> MVSSKKFNQVDKGRGMISENYIEPAFLLPDLIEIQRSSFRWFLEEGLIEELNSFSPITDYTGKLELHFLGHNYKLKEPKYSVEEAKRRDSTYAVQMYVPTRLLNKETGDIKEQEVFIGDLPLMTDRGTFIINGAERVIVNQIVRSPGVYYKSEIDKNGRRTYSASLIPNRGAWLKFETDRNDLVWVRIDKTRKLSAQVLLKALGLSDNEIFDALRHPEYFQKTIEKEGQFSEEEALMELYRKLRPGEPPTVLGGQQLLDSRFFDPKRYDLGRVGRYKLNKKLRLSVPDTVRVLTSGDILAAVDYLINLEYDIGSIDDIDHLGNRRVRSVGELLQNQVRVGLNRLERIIRERMTVSDAEVLTPASLVNPKPLVAAIKEFFGSSQLSQFMDQTNPLAELTHKRRLSALGPGGLTRERAGFAVRDIHPSHYGRICPIETPEGPNAGLIGSLATHARVNQYGFLETPFRPVENGRVRFDQPAAYMTADEEDDLRVAPGDIPVDENGYIIGPQVPVRYRQEFSTTTPEQVDYVA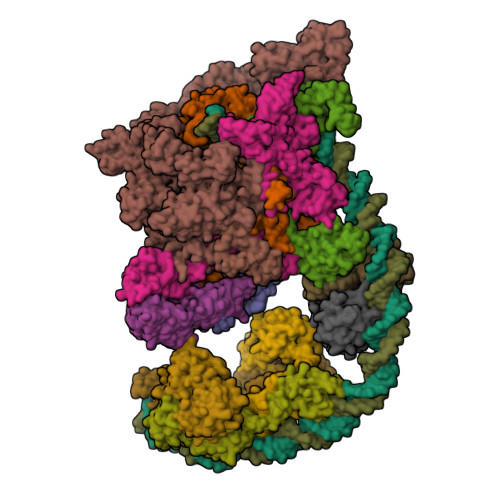VSPVQIVSVATSMIPFLEHDDANRALMGSNMQRQAVPLLKPERPLVGTGLEAQGARDSGMVIVSRTDGDVVYVDATEIRVRVSGQLPTASGKSTDNGQLTSQKGQEIRYTVSKYQRSNQDTCLNQKPLVRIGERVVAGQVLADGSSTEGGELALGQNIVVAYMPWEGYNYEDAILISERLVQDDIYTSIHIEKYEIEARQTKLGPEEITREIPNVGEDALRQLDEQGIIRIGAWVEAGDILVGKVTPKGESDQPPEEKLLRAIFGEKARDVRDNSLRVPNGEKGRVVDVRLFTREQGDELPPGANMVVRVYVAQKRKIQVGDKMAGRHGNKGIISRILPIEDMPYLPDGSPVDIVLNPLGVPSRMNVGQVFECLLGWAGHTLGVRFKITPFDEMYGEESSRRIVHGKLQEARDETGKDWVYNPDDPGKIMVYDGRTGEAFDRPVTIGVAYMLKLVHLVDDKIHARSTGPYSLVTQQPLGGKAQQGGQRFGEMEVWALEAFGAAYTLQELLTVKSDDMQGRNEALNAIVKGKAIPRPGTPESFKVLMRELQSLGLDIAVHKVETQADGSSLDVEVDLMADQLARRTPPRPTYESLSRESLDDDE;> MIFRNRVVDKGQLRNLISWAFTHYGTARTAVMADKLKDLGFRYATRAGVSISVDDLMVPPSKRSLLEAAEEEIRATEVRYQRGEITEVERFQKVIDTWNGTSEALKDEVVTHFKQTNPLNSVYMMAFSGARGNISQVRQLVGMRGLMADPQGEIIDLPIKTNFREGLTVTEYIISSYGARKGLVDTALRTADSGYLTRRLVDVSQDVIIREIDCGTTRGIPVRPMTEGSKTLIKLSTRLLGRVVGEDVIHPKTKEVIAPRNTPISDDLAKEIEKAGVAEVVVRSPLTCEAARSVCQHCYGWSLAHAKMVDLGEAVGIIAAQSIGEPGTQLTMRTFHTGGVFTGEVAQQVRSKMDGTIKLPRKLRTRTHRTRHGEDALFVESNGIMILEPRKEGSETPAPQEIHVTQGSTIYIVDGQQVKKGQLLAEVALGGRTTRTNTEKAVKDVASDLAGEVKFAEVVPEQKTDRQGNTTTTAARGGLIWILSGEVYNLPPGAELVVKNGDRVETNGVLAETKLTTIHGGVVRLPEATPGKSTREIEIITASVVLDQATVTVQSSQGRNNYLITTGNNQVFNLRATPGTKVQNGQVVAELIDDRYRTTTGGFLKFAGVEVQKKGKAKLGYEVVQGGTLLWIPEETHEVNKDISLLLVEDGQYVEAGTEVVKDIFCQNSGVVEVTQKNDILREVVVKPGELLMVDDPEAVIGRDNTLLQPGEELLGQVATELRYIQYVESPEGPALLSRPVVEFAVPSNPDVPSTTSVSQQTGRSIQMRAVQRLPYKDSERVKSVEGVELLRTQLVLEIEQEGEQEHNASPLAADIELIPDLEDADVQRLQLVILESLVLRRDIAADATQGSTQTSLEVKDGDTIVPGSVVARTQILSKEGGIVRGVQKGSEAVRRCLVLRHSDMATLNISAKPKVKAGDLIVAGTELAPGIFAEESGQIVGVKNAGESTTTQDAALSTQNYAVTIRAGRPYRVSPGAVLQIEDGDLVQRGDNLVLLVFERAKTGDIIQGLPRIEELLEARKPKEACILAKRGGEVKVVYGDGDEAIAIKVIESNGVVTDYPLGPGQNLAMPDGSVVPAGQPLSDGPSNPHEILEVFFSLGSEDGVYACASHALQKVQTFLVNEVQMVYQSQGIDIADKHIEVIVRQMTNKVRIDDGGDTTMLPGELVELRQVEQVNEAMAITGGARAQYTPVLLGITKASLNTDSFISAASFQETTRVLTEAAIEGKSDWLRGLKENVIIGRLIPAGTGYNTYDEPGMLEDYSTLETTSVLDETDDPLDMVLDDRTARAYNLDSPGLAETGFNNRRSILDDDELIADEIHDLVEAEVEVDDEVDDDYEDDDEDDDDYED;>[2x]MVAQFQIECVESNTEESRNHYSKFILEPLERGQGTTVGNALRRVLLSNLEGTAVTAVRIAGVSHEFATVPGVREDVLEIIMRMKEVILKSYSSQAQIGRLLVNGPTTITASHFDLPSEVEVIDPTQYVATIAEGGKLEMEFRIERGKGYRTVERGREEATSLDFLQIDSIFMPVRKVNYSVEEVRADGSIPKDRLLLEVWTNGSISPQEALSSAAGILVDLFNPLKDISLEPTDTN;> MRPAQTNQFDYVKIGLASPERIRQWGERTLPNGQVVGEVTKPETINYRTLKPEMDGLFCERIFGPAKDWECHCGKYKRVRHRGIVCERCGVEVTESRVRRHRMGYIKLAAPVAHVWYLKGIPSYISILLDMPLRDVEQIVYFNSYVVLSPGNAETLTYKQLLSEDQWLEIEDQIYSEDSQLQGVEVGIGAEALLRLLADINLEQEAESLREEIGSAKGQKRAKLIKRLRVIDNFIATGSKPEWMVMTVIPVIPPDLRPMVQLDGGRFATSDLNDLYRRVINRNNRLARLQEILAPEIIVRNEKRMLQEAVDALIDNGRRGRTVVGANNRPLKSLSDIIEGKQGRFRQNLLGKRVDYSGRSVIVVGPKLKIHQCGLPREMAIELFQPFVINRLIRSGMVNNIKAAKKLISRNDPSVWDVLEEVIEGHPVMLNRAPTLHRLGIQAFEPILVEGRAIQLHPLVCPAFNADFDGDQMAVHVPLSLESQAEARLLMLASNNILSPATGRPIITPSQDMVLGAYYLTAENPGATKGAGKYFASLDDVIMAFQQEQIDLHAYVYVRFDGDVESDQPDTEPVKVTTNEDGSRTVLYKYRRVREDAQGNVISQYIYTTPGRVIYNKAIQEALAS;> MLKRSKFETTQSQIMHRAEDLISAASNRYRITVQVANRAKRRRYEEFESAEDAMMKPVLRAIIEMSDELTQPEIIGEI;> MNQANNVLDSIYQPDLEIMNQPEIELDDLLIEEDEDLLLADDGDIDEFLEPQTDEDDAKSGKAAKSRRRTQSKKKHYTEDSIRLYLQEIGRIRLLRADEEIELARKIADLLELERVRERLSEKLERDPRDSEWAEAVQLPLPAFRYRLHIGRRAKDKMVQSNLRLVVSIAKKYMNRGLSFQDLIQEGSLGLIRAAEKFDHEKGYKFSTYATWWIRQAITRAIADQSRTIRLPVHLYETISRIKKTTKLLSQEMGRKPTEEEIATRMEMTIEKLRFIAKSAQLPISLETPIGKEEDSRLGDFIESDGETPEDQVSKNLLREDLEKVLDSLSPRERDVLRLRYGLDDGRMKTLEEIGQIFNVTRERIRQIEAKALRKLRHPNRNSVLKEYIR;>[4x]MRLEQLQAFLAIAETGSFQKAASKCGVTQSTISRQIQSLEADLGLELFHRTNHSKLTLGGERLLPRARKICLEWETATQELGDLIAGKQPELCIAAIHSLCGSYLPPVLQKFCRDYPEVQLRVTSLGSDRALKVLKDGLVDLAIVMNNRFLTTGRDMVVEVLYDEPIELLTAANHPLAAYERVPWSELVRYPQVVFKDGYGMQRLVQEKFERLEATLQAALEVNTLDAFRGVVRQGELIALLPSSALVEARLDPTLAVRPLANSALPENSGLTRRVVMVTTQDRLQIPPIKHFWQLVRENIPPIVERQRSAS;>MIVTQDKALANVFRQMATGAFPPVVETFERNKTIFFPGDPAERVYFLLKGAVKLSRVYEAGEEITVALLRENSVFGVLSLLTGNKSDRFYHAVAFTPVELLSAPIEQVEQALKENPELSMLMLRGLSSRILQTEMMIETLAHRDMGSRLVSFLLILCRDFGVPCADGITIDLKLSHQAIAEAIGSTRVTVTRLLGDLREKKMISIHKKKITVHKPVTLSRQFT[2x]> MASTSGTINV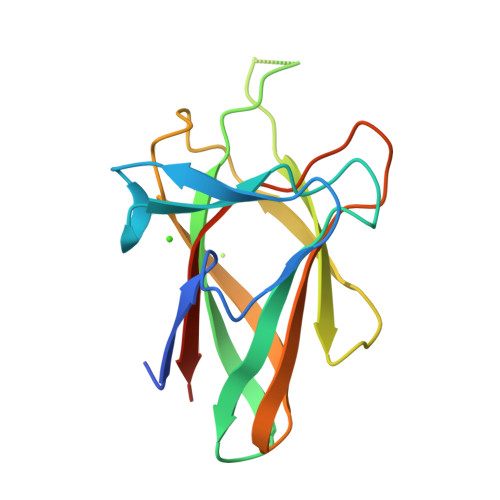YEAEDPANTLGGAAVRQRDNAASGGQYVGWIGNGSNNYLQFNNVYVPQAGTYRMVVQFANAEVFGQHSYNNNVVDRYCSISVNGGPEKGHYFFNTRGWNTYRTDIIDVYLNAGNNTIRFYNGTSGSYAPNIDKIAIAALEHHHHHH7-[2-METHOXY-1-(METHOXYMETHYL)ETHYL]-7H-PYRROLO[3,2-F] 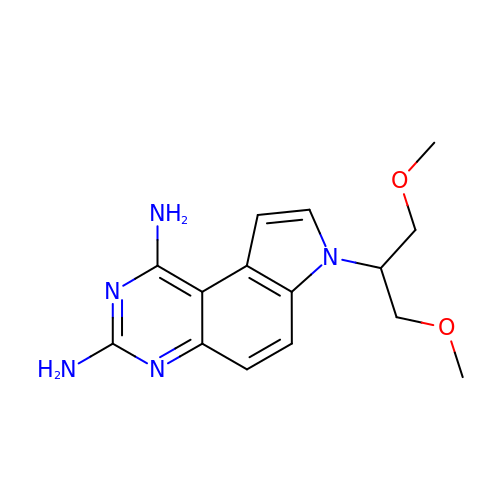QUINAZOLINE-1,3-DIAMINE | C15 H19 N5 O2 | MQTGHZCEDQNMOZ-UHFFFAOYSA-N> GPAPNEEFVGDMRIVNVNLSNIDILKKHETFKKYFDFTLTGPRYNGNIAEFAMIWKIKNPPLNLLGVFFDDGTRDDEDDKYILEELKQIGNGAKNMYIFWQYEQK;> GPVLEATMICIDNSEWMRNGDYSPSRLQAQTEAVNLLCGAKTQSNPENTVGILTMAGKGVRVLTTPTSDLGKILACMHGLDVGGEINLTAAIQIAQLALKHRQNKNQRQRIIVFAGSPIKYEKKALEIVGKRLKKNSVSLDIVNFGEDDDEEKPQKLEALLTAVNNNDGSHIV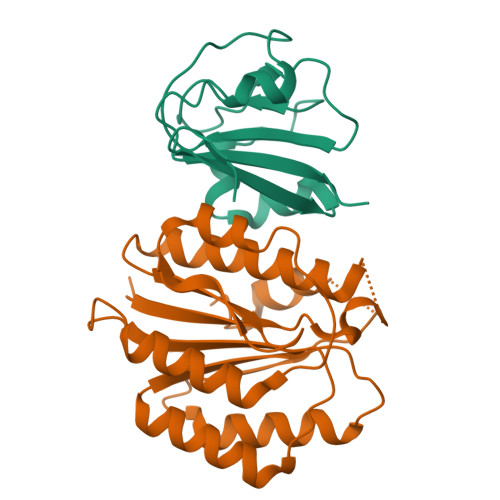HVPSGANALSDVLLSTPVFTG> IIGGREVIPHSRPYMASLQRNGSHLCGGVLVHPKWVLTAAHCLAQRMAQLRLVLGLHTLDSPGLTFHIKAAIQHPRYKPVPALENNLALLQLDGKVKPSRTIRPLALPSKRQVVAAGTRCSMAGWGLTHQGGRLSRVLRELDLQVLDTRMCNNSRFWNGSLSPSMVCLAADSKDQAPCKGDSGGPLVCGKGRVLAGVLSFSSRVCTDIFKPPVATAVAPYVSWIRKVTGRSALEHHH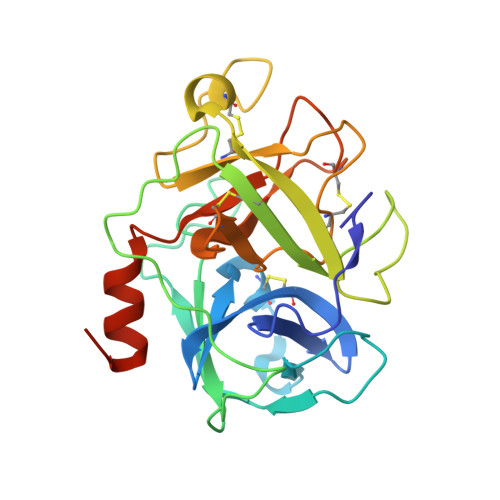HHH>[2x]MTPSHPARPSRSGILVFDVNETLLDLTSLSPLFERVFGDAKVLREWFPELILYSQTLTLTGLYRPFGEIAAAVFEMVAANHQAKVTPDDIAELKTRLTSMPAYPDVAPALT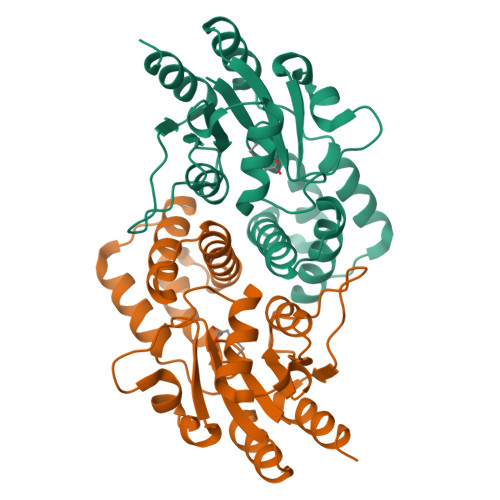RLQDAGFRLVTLTNSAPSPAPSPLEKAGIASFFEAHLTVHSSQRFKPHPSVYDSTAETLGAKPEELCMIACHIWATIGAQARGWRGGFVARPHNTPLTLAEVPQPDFIGRDMGELADQLIASLTA> MGHHHHHHAENLYFQGHMEITTDSLLALLGSEKVKIIDVR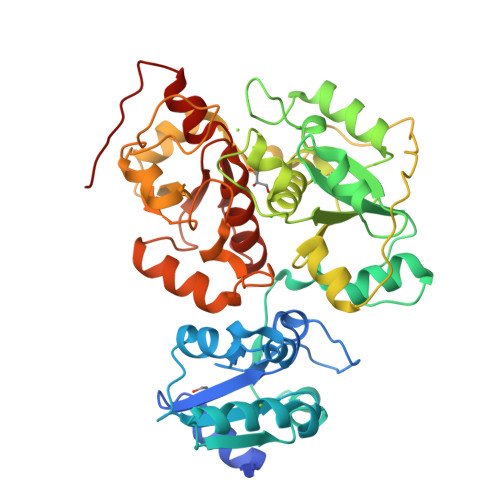SADAYNGWRMRGEVRGGHIKGAKSLPAKWLTDPEWLNIVRFKQIRPEDAIVLYGYTPEECEQTATRFKENGYNNVSVFHRFHPDWTGNDAFPMDRLEQYNRLVPAEWVNGLISGEEIPEYDNDTFIVCHAHYRNRDAYLSGHIPGATDMDTLALESPETWNRRTPEELKKALEEHGITASTTVVLYGKFMHPDNADEFPGSAAGHIGAIRLAFIMMYAGVEDVRVLNGGYQSWTDAGFAISKDDVPKTTVPEFGAPIPSRPEFAVDIDEAKEMLQSEDSDLVCVRSYPEYIGEVSGYNYIAAAGRIPGAIFAECGSDAYHMENYRNHDHTTREYHEIEDIWAKSGIIPKKHLAFYCGTGWRGSEAWFNALLMGWPRVSVYDGGWFEWSNDPENPYETGVPK>[3x]MHHHHHHENLYFQGHMKKWGDMFTWGVSTSSYQIE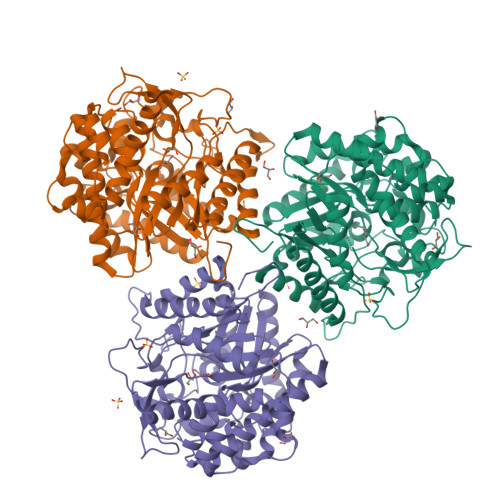GAANQGGRGPSIWDTFSKIPGAVANGDNGDVACDHYHRYNEDLDLMKWLGVGAYRFSIAWPRVIPSGYGALNKEGMDFYDRLIDGALERGITPWPTLYHWDLPQSLQDKGGWNNRDCAYWFAEYSQKMAEAFSDRLKNWITINEPFCSAWLGHLYGVMAPGIKDLKTGINASHHLLLGHGLATKAIREVSSELKVGITLNFTPAITLGESSEDKLAVELADGFDNRWFGDPVFKAKYPEDIVKAFGKEVPIHPGDMEIISTPLDYLGLNYYFRQTVEYDATAKPLPYKQVTAPNVERTGMGWEVHAQSFTELLERVSKEYKPKEIFITENGSAWDDEVVDGKVDDPNRVSYLERHLDAMFAAKNKGVPISGYFAWSLIDNFEWAYGYAKRFGIIYVDYQTQKRIPKSSAYYYQKRIKES> MPEITRRRALTAAAAVAATASAAVTLAAPAASAAGHHEPAAPESFDEVYKGRRIQGRPAGGGAHHHEHGGGYEVFVDGVQLHVMRNADGSWISVVSHYDPVPTPRAAARA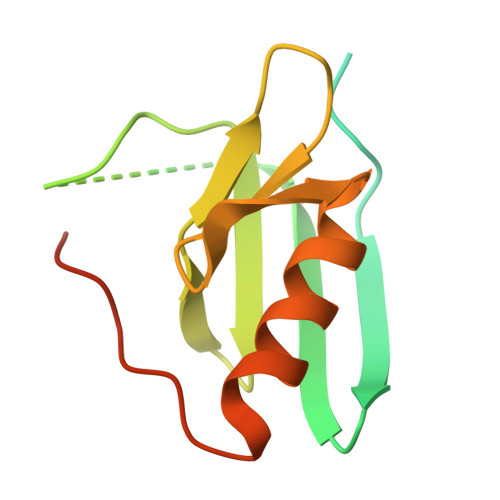AVDELQGAPLLPFPANLEHHHHHH> MSEEKSRNGPARLKLVLGGATLGVVALATVAFGMKYTDQRPFCTSCHIMNPVGVTHKLSGHANISCNDCHAPHNLLAKLPFKA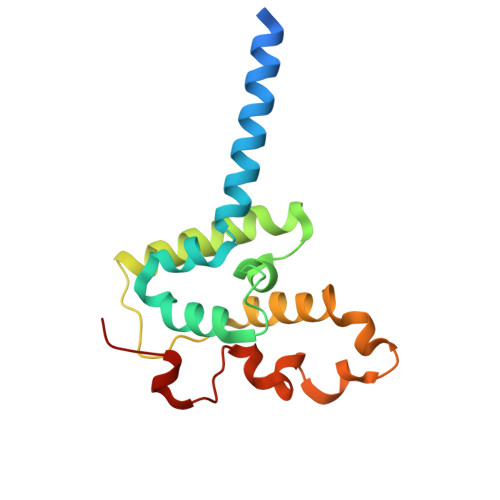IAGARDVYMNTLGHPGDLILAGMETKEVVNANCKACHTMTNVEVASMEAKKYCTDCHRNVQHMRMKPISTREVADE>TIEKRYDFVFLFDVQDGNPNGDPDAGNLPRIDPQTGEGLVTDVCLKRKVRNFIQMTQNDEHHDIFIREKGILNNLIDEAHEQENVKGKEKGEKTEAARQYMCSRYYDIRTFGAVMTTGKNAGQVRGPVQLTFSRSIDPIMTLEHSITRMAVTNEKDASETGDNRTMGRKFTVPYGLYRCHGFISTHFAKQTGFSENDLELFWQALVNMFDHDHSAARGQMNARGLYVFEHSNNLGDAPADSLFKRIQVVKKDGVEVVRSFDDYLVSVDDKNLEETKLLRKLGG[7x];>[2x]MILHALTQYYQRKAESDGGIAQEGFENKEIPFIIVIDKQGNFIQLEDTRELKVK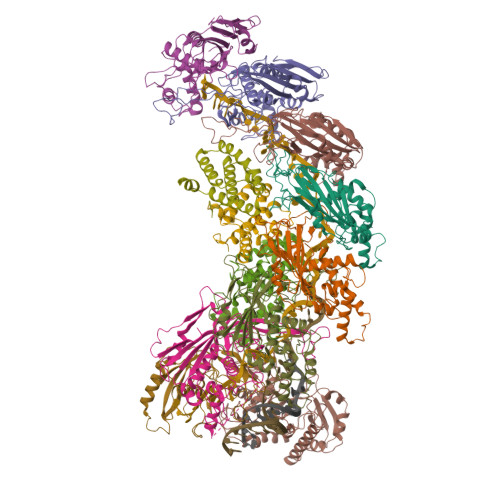KKVGRTFLVPKGLGRSGSKSYEVSNLLWDHYGYVLAYAGEKGQEQADKQHASFTAKVNELKQALPDDAGVTAVAAFLSSAEEKSKVMQAANWAECAKVKGCNLSFRLVDEAVDLVCQSKAVREYVSQANQTQSDNAQKGICLVTGKAAPIARLHNAVKGVNAKPAPFASVNLSAFESYGKEQGFAFPIGEQAMFEYTTALNTLLAGENRFRIGDVTTVCWGAKRTPLEESLASLINGGGKDKPDAHIDAVKALYKSLYNGQYCKPDGEDKFYLLGLSPNSARIVVRFWHETTVAALSESIAAWYDDLQMVRGENSPYPEYMPLPRLLGNLVLDGKMENLPSDLIAQITDAALNNRVLPVSLLQAALRRNKAEQKITYGRASLLKAYINRAIRAGRLKNMKELTMGLDRNRQDIGYVLGRLFAVLEKIQAEANPGLNATIADRYFGSASSTPIAVFGTLMRLLPHHLNKLEFEGRAVQLQWEIRQILEHCQRFPNHLNLEQQGLFAIGYYHETQFLFTKDALKNLFNEA;>[2x]GLDRNRQDIGYVLGRLFAVLEKIQAEANPGLNATIADRYFGSASSTPIAVFGTLMRLLPHHLNKLEFEGRAVQLQWEIRQILEHCQRFPNHLNLEQQGLFAIGYYHETQFLFTKDALKNLFNEA;> RFILEISGDLACFTRSELKVERVSYPVITPSAARNILMAILWKPAIRWKVLKIEILKPIQWTNIRRNEVGTKMSERSGSLYIEDNRQQRASMLLKDVAYRIHADFDMTSEAGESDNYVKFAEMFKRRAKKGQYFHQPYLGCREFPCDFRLLEKAEDGLPLEDITQDFGFMLYDMDFSKSDPRDSNNAEPMFYQCKAVNGVITVPP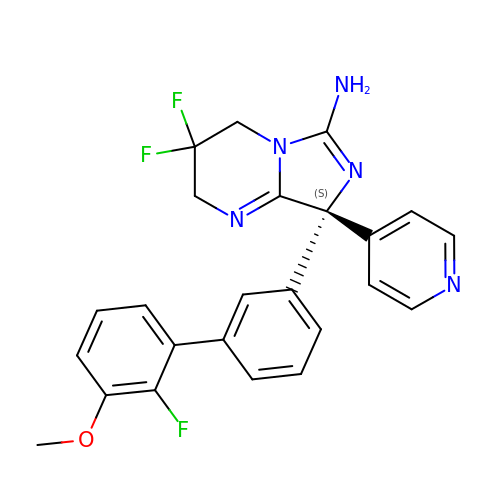(8S)-3,3-DIFLUORO-8-(2'-FLUORO-3'-METHOXYBIPHENYL-3-YL)-8-PYRIDIN-4-YL-2,3,4,8-TETRAHYDROIMIDAZO[1,5-A]PYRIMIDIN-6-AMINE | C24 H20 F3 N5 O | RECVUKARQVUVBY-XMMPIXPASA-N> GPLGSRQWALEDFEIGRPLGKGK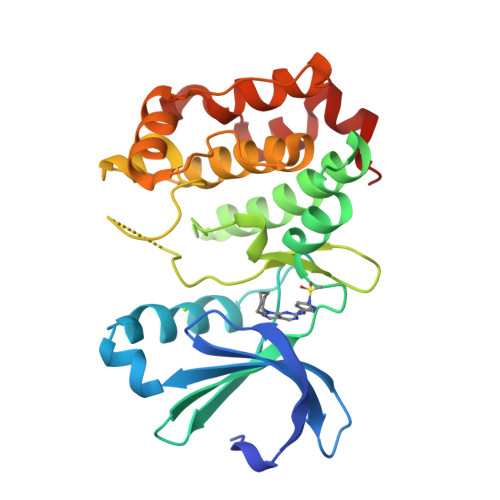FGNVYLAREKQSKFILALKVLFKAQLEKAGVEHQLRREVEIQSHLRHPNILRLYGYFHDATRVYLILEYAPLGTVYRELQKLSKFDEQRTATYITELANALSYCHSKRVIHRDIKPENLLLGSAGELKIADFGWSVHAPSSRRDDLCGTLDYLPPEMIEGRMHDEKVDLWSLGVLCYEFLVGKPPFEANTYQETYKRISRVEFTFPDFVTEGARDLISRLLKHNPSQRPMLREVLEHPWITANSSKPS> MGSLKVDVEALENSAGATYIRKKGGKVTGDSQPKEQGQGDLKKKKKKKKGKLPKNYDPKVTPDPERWLPM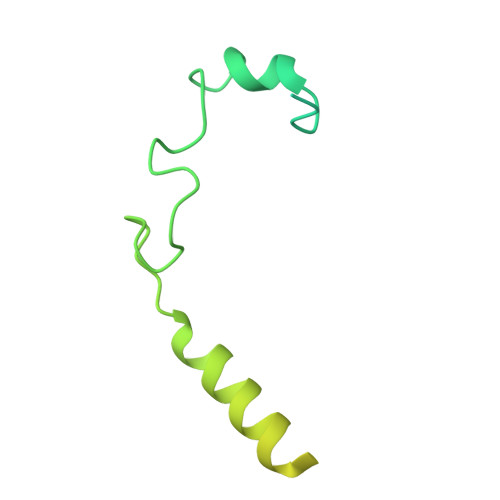RERSYYRGRKKGKKKDQIGKGTQGATAGASSELDASKTVSSPPTSPRPGSAATVSASTSNIIPPRHQKPAGAPATKKKQQQKHHHHHH> MRALFYKDGKLFTDNNFLNPVSDNNPAYEVLQHVKIPTHLTDVVVYGQTWEEALTRLIFVGSDSKGRRQYFYGKMHVQNRNAKRDRIFVRVYNVMKRINSFINKNIKKSSTDSNYQLAVFMLMETMFFIRFGK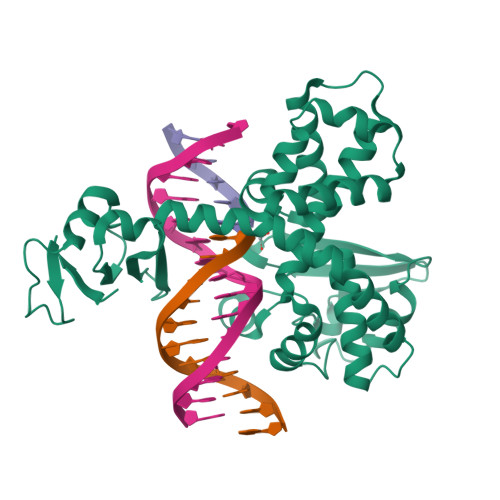MKYLKENETVGLLTLKNKHIEISPDKIVIKFVGKDKVSHEFVVHKSNRLYKPLLKLTDDSSPEEFLFNKLSERKVYESIKQFGIRIKDLRTYGVNYTFLYNFWTNVKSISPLPSPKKLIALTIKQTAEVVGHTPSISKRAYMATTILEMVKDKNFLDVVSKTTFDEFLSIVVDHVKSSTDG>[2x]MSDGVEVKNITFKLGMYL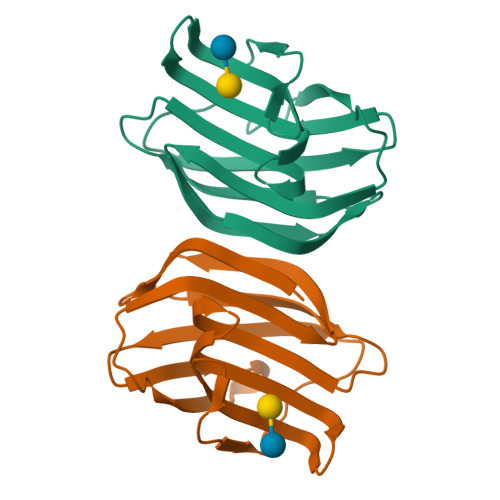TVGGVVNSNAKRFSINVGESTDSIALHIDHRFSYGADQNTIVLNSMVDDGWQQEQRSKNFPFTAGEHFQITITFDIDTFYIQLPDGHKVEFPNRHGDEAFNFIYLAGDARLTFVRLE> MYIGKPIKRIEDLRLITGKGAYVDDIELPGTLFVAFVRSKYPHARIKVKKEEGIFTGEDINPGKDFPIATKETTYVGQPIAIVIAKDRYEAYDLIESVEVEYEELDYVLDPEKALEDKVKVHSGLSSNIYYHERWKGGDVEKAFKEADLTISDTLINQRVIASPLETRGALAYFDGNKLTFYSSTQSAHYLRRNLVDFLGFENIRVIQPDVGGAFGSKIIAHPEEYALAKLALMLRKPLKWVPTRTEEFISAGHGRDKKLKFEVAVKKDGTILGIRGTLIANLGAPYPDANDDESGNVKSTVRMLPGIYKIIGADIDAYAVHTNITPTQSYRGAGRPEGIYFIERIVNIVADELGIDQYEIRLKNAIDTLPYTNIFGVTYDSGNVKKLLEIGKKYYDELKKEDGCVGVSSYIEITAFGPWEVARISVKYDGKITLVTGTGPHGQGDATAFAQIAADVLELPIEKIEVRWGDTEIIEDGIGTWGSRTVTIGGSAVLLASQKLKDKLIEIGAKILNADKEEVEYKEGNVTHKKNGNKVTFNEIVKNAFKMGESLDTTAIYNVKQPPTTPYGVHLALVKVDGTGKVFVKKYVAVDDVGTVINPLLAEGQAIGGIVQGMAQALLEGAFFDENGQLLTTNFQDYPIPTAVEIPEKIDWYYEILGKSPHPTGSKGIGEAGAIAATPTIINAVEQCIKKRITKMPVKFEELVS;> MYPPKFGYVIPDNLNEALEFLEEHQDARPLAGGHSLIPMLKLRLIRPSYIVEIRRFSNLSYITKDGNLYKIGALTTHYNISKSSIPLLSETASNIGDPQVRNMGTIGGSISHLDPSADYPAALIAMDAKVKITSRKGDRVVNFKSFAKDMFTPDLNPGELVTEIQVPTFEGYKFSYQKLERRAGDFAIVGVALLLKLSGDVIEDVRIGLTAVNNVAVRAKGAEEELLGKRLNDEIIEKAATRAMESANPTSDLRGSAEYKKKMVKV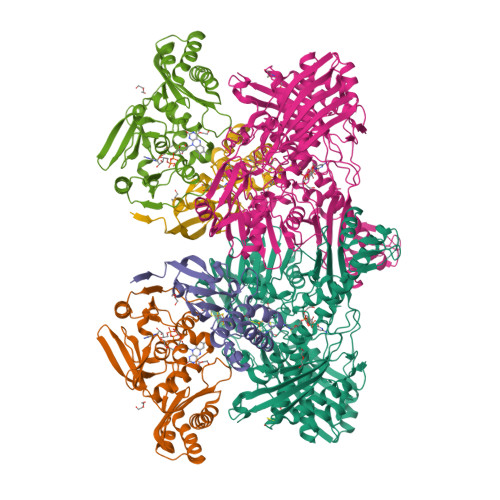LTKRAIITALKR;> MKIINSDQKVKITLKINGEKYETEVEPRRLLVHVLRELGFTGVHIGCDTSNCGACTVIMNGKSVKSCTVLAVEADGAEILTVEGLAKDGKLHPIQEAFWENHALQCGYCTPGMIMEAYWLLREKPNPTEEEIREGISGNLCRCTGYQNIVKAIKAAAEKLSQTPYQHQ>MRMTWNFHQYYTNRNDGLMGKLVLTDEEKNNLKALRKIIRLRTRDVFEEAKGIAKAVKKSALTFEIIQEKVSTTQIKHLSDSEQREVAKLIYEMDDDARDEFLGLTPRFWTQGSFQYDTLNRPFQPGQEMDIDDGTYMPMPIFESEPKIGHSLLILLVDASLKSLVAENHGWKFEAKQTCGRIKIEAEKTHINVPMYAIPKDEFQKKQIALEANRSFVKGAIFESYVADSITDDSETYELDSENVNLALREGDRKWINSD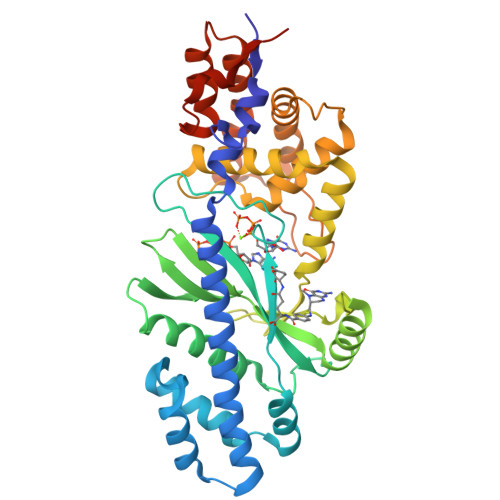PKIVEDWFNDSCIRIGKHLRKVCRFMKAWRDAQWDVGGPSSISLMAATVNILDSVAHDASDLGETMKIIAKHLPSEFARGVESPDSTDEKPLFPPSYKHGPREMDIMSKLERLPEILSSAESADSKSEALKKINMAFGNRVTNSELIVLAKALPAFAQELEHHHHHH[2x]>ASSVNELENWSKWMQPIPDNIPLARISIPGTHDSGTFKLQNPIKQVAGMTQEYDFRYQMDHGARIFDIRGRLTDDNTIVLHHGPLYLYVTLHEFINEAKQFLKDNPSETIIMSLKKEYEDMKGAEGSFSSTFEKNYFVDPIFLKTEGNIKLGDARGKIVLLKRYSGSNESGGYNNFYWPDNETFTTTVN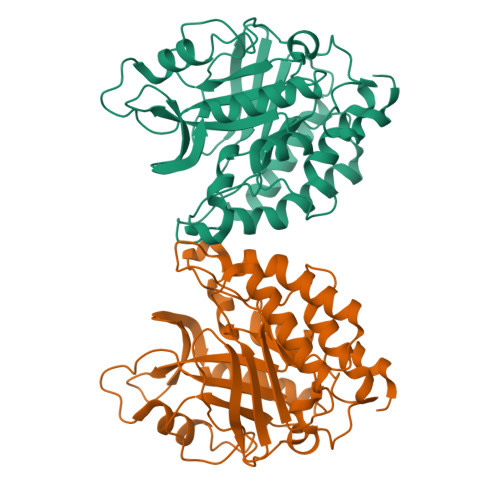QNVNVTVQDKYKVNYDEKVKSIKDTMDETMNNSEDLNHLYINFTSLSSGGTAANSPYYYASYINPEIANDIKQKNPTRVGWVIQDYINEKWSPLLYQEVIRANKSLI[2x]> MERYENLFAQLNDRREGAFVPFVTLGDPGIEQSLKIIDTLIDAGADALELGVPFSDPLADGPTIQNANLRAFAAGVTPAQCFEMLAIIREKHPTIPIGLLMYANLVFNNGIDAFYARCEQVGVDSVLVADVPVEESAPFRQAALRHNIAPIFICPPNADDDLLRQVASYGRGYTYLLSRSGVTGAENRGALPLHHLIEKLKEYHAAPALQGFGISSPEQVSAAVRAGAAGAISGSAIVKIIEKNLASPKQMLAELRSFVSAMKAASRA;> TTLLNPYFGEFGGMYVPQILMPALNQLEEAFVSAQKDPEFQAQFADLLKNYAGRPTALTKCQNITAGTRTTLYLKREDLLHGGAHKTNQ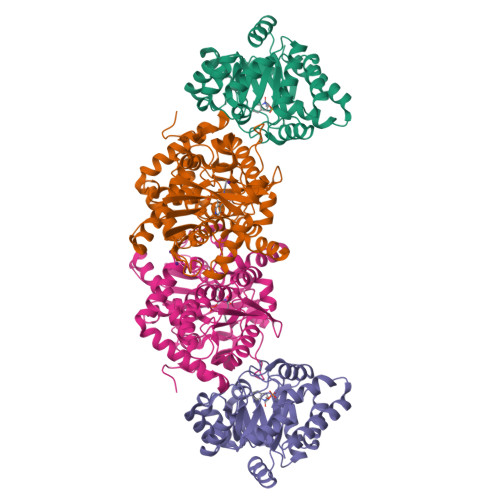VLGQALLAKRMGKSEIIAETGAGQHGVASALASALLGLKCRIYMGAKDVERQSPNVFRMRLMGAEVIPVHSGSATLKDACNEALRDWSGSYETAHYMLGTAAGPHPYPTIVREFQRMIGEETKAQILDKEGRLPDAVIACVGGGSNAIGMFADFINDTSVGLIGVEPGGHGIETGEHGAPLKHGRVGIYFGMKAPMMQTADGQIEESYSISAGLDFPSVGPQHAYLNSIGRADYVSITDDEALEAFKTLCRHEGIIPALESSHALAHALKMMREQPEKEQLLVVNLSGRGDKDIFTVHDILKARGEI> STPIQQLLEHFLRQLQRKDPHGFFAFPVTDAIAPGYSMIIKHPMDFGTMKDKIVANEYKSVTEFKADFKLMCDNAMTYNRPDTVYYKLAKKILHAGFKMM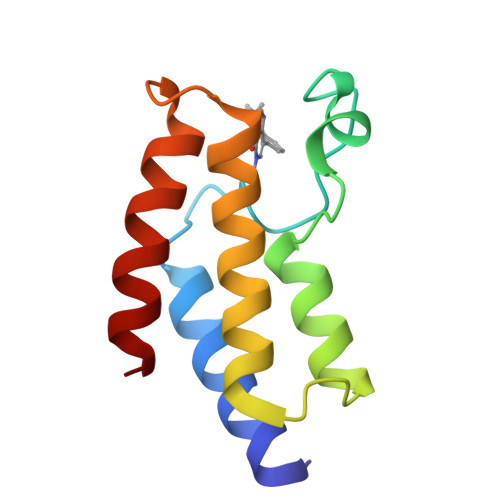S>MRIGITYTVLRREEMAIKERAGEFGEVVMLHEDDLLFPGNYDLDVVIIRNVSHFKALYTARLFESEGIPTVNSSRLIFEAGDKLFATLRLAGKVPVPEWKAALSEGGALRVPDSLGYPLVSKPVFGSWGRLLAKVNDRDSLEAVLEHRKWMKNPLYGIHYFQEFVEKPGRDIRSYVIGGEFVGAIYRYSNHWITNTARGGKAEPCSDPEVEELSVKAWEAFGEGALAIDIFESEKGLLVNEVNPNMEFKNAARVTGADMAGKLVEYAVEVAKT[8x];>MVECPVCGSEIEIGEVELHQIVECPVCGAELEVVSLEPLTLEE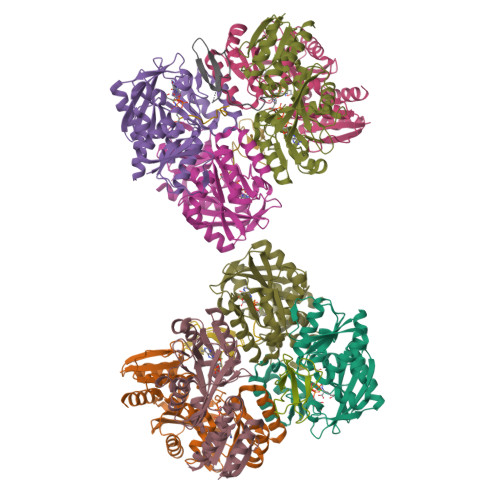LPEVEEDWGE[6x]> ASTPQKFYLTPPQVNSILKANEYSFKVPEFDGKNVSSVLGFDSNQLPANAPIEDRRSAATCLQTRGMLLGVFDGHAGCACSQAVSERLFYYIAVSLLPHETLLEIENAVESGRALLPILQWHKHPNDYFSKEASKLYFNSLRTYWQELIDLNTGESTDIDVKEALINAFKRLDNDISLEAQVGDPNSFLNYLVLRVAFSGATACVAHVDGVDLHVANTGDSRAMLGVQEEDGSWSAVTLSNDHNAQNEREVERLKLEHPKNEAKSVVK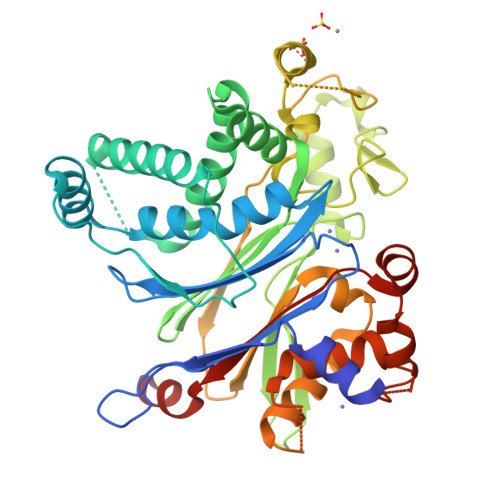QDRLLGLLMPFRAFGDVKFKWSIDLQKRVIESGPDQLNDNEYTKFIPPNYYTPPYLTAEPEVTYHRLRPQDKFLVLATDGLWETMHRQDVVRIVGEYLTGMHHQQPIAVGGYKVTLGQMHGLLTERRAKMSSVFEDQNAATHLIRHAVGNNEFGAVDHERLSKMLSLPEELARMYRDDITIIVVQFNSHVVGAYQNQEQ>[2x]MACGLVASNLNLKPGECLRVRGEVAPDAKSFVLNLGKDSNNLCLHFNPRFNAHGDANTIVC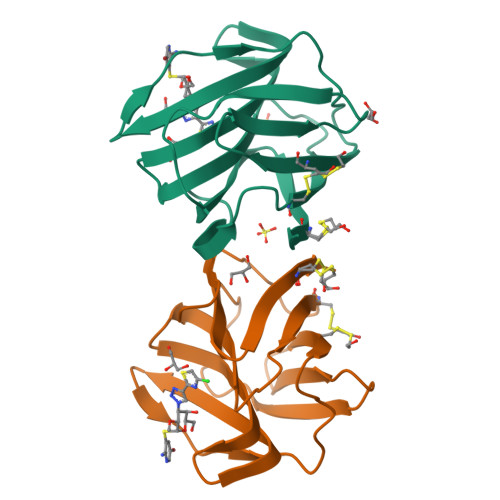NSKDGGAWGTEQREAVFPFQPGSVAEVCITFDQANLTVKLPDGYEFKFPNRLNLEAINYMAADGDFKIKCVAFD> MTNEQVIELVRVLLGGITTEEISDQTIIFFWTKWKLTYDLDNRPEKIPAALYNTVVDCVRWLIVQEVSSGNSSIRERFEKIGDETISVKGGSSWESWKDFLDWLELNPDYIDPSLAFNSSLVIIGGVRKDEFFRVKNNPNSYNGFMEQGVYPTPAIPKQSAW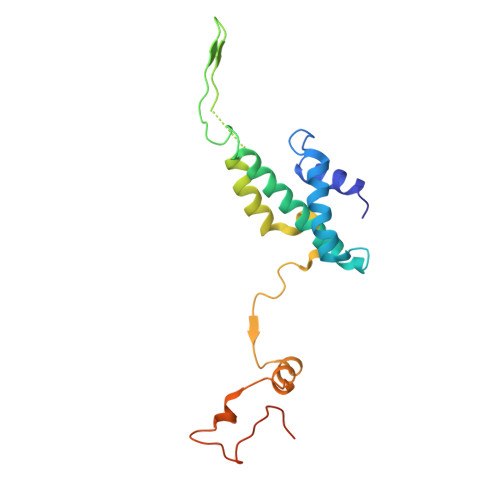PCTAARRSPWMVR> MSSSAPKYTTFQGSQNFRLRIVLATLSGKPIKIEKIRSGDLNPGLKDYEVSFLRLIESVTNGSVIEISYTGTTVIYRPGIIVGGASTHICPSSKPVGYFVEPMLYLAPFSKKKFSILFKGITASHNDAGIEAIKWGLMPVMEKFGVRECALHTLKRGSPPLGG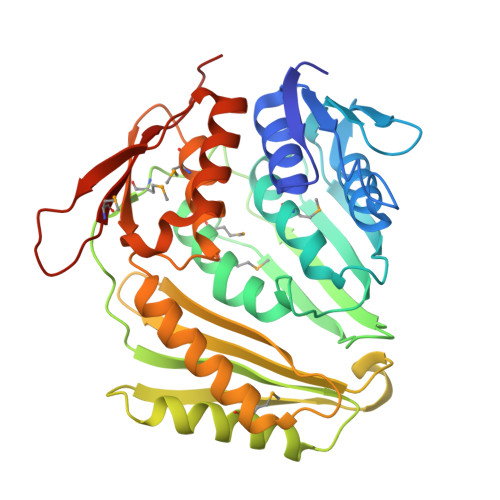GEVHLVVDSLIAQPITMHEIDRPIISSITGVAYSTRVSPSLVNRMIDGAKKVLKNLQCEVNITADVWRGENSGKSPGWGITLVAQSKQKGWSYFAEDIGDAGSIPEELGEKVACQLLEEISKSAAVGRNQLPLAIVYMVIGKEDIGRLRINKEQIDERFIILLRDIKKIFNTEVFLKPVDEADNEDMIATIKGIGFTNTSKKIA> MADGQVAELLLRRLEASDGGLDSAELAAELGMEHQAVVGAVKSLQALGEVIEAELRSTKHWELTAEGEEIAREGSHEARVFRSIPPEGLAQSELMRLPSGKVGFSKAMSNKWIRVDKSAADGPRVFRVVDSMEDEVQRRLQLVRGGQAEKLGEKERSELRKRKLLAEVTLKTYWVSKGSAFSTSISKQETELSPEMISSGSWRDRPFKPYNFLAHGVLPDSGHLHPLLKVRSQFRQIFLEMGFTEMPTDNFIESSFWNFDALFQPQQHPARDQHDTFFLRDPAEALQLPMDYVQRVKRTHSQGGYGSQGYKYNWKLDEARKNLLRTHTTSASARALYRLAQKKPFTPVKYFSIDRVFRNETLDATHLAEFHQIEGVVADHGLTLGHLMGVLREFFTKLGITQLRFKPAYNPYTEPSMEVFSYHQGLKKWVEVGNSGVFRPEMLLPMGLPENVSVIAWGLSLERPTMIK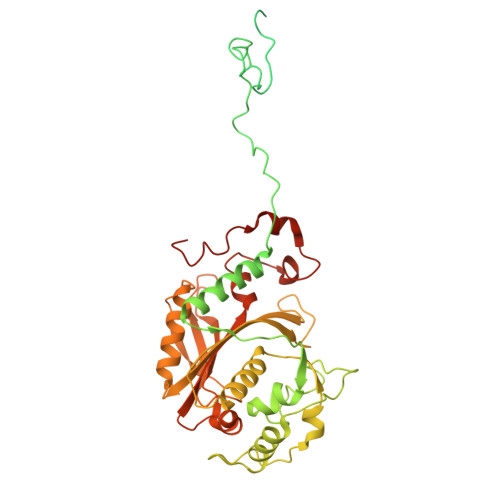YGINNIRELVGHKVNLQMVYDSPLCRLDAEPRPPPTQEAA> EQRITLKDYAMRFGQTKTAKDLGVYQSAINKAIHAGRKIFLT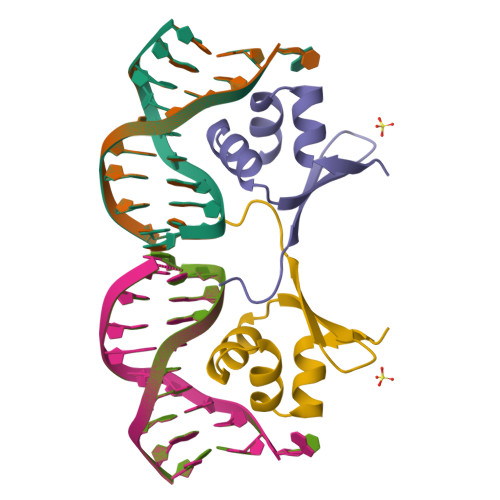INADGSVYAEEVKPFPSN>[24x]MSQSGEDLHSPTYLSWRKLQLSRAKLKASSWTSALLSGFAMVAMVEVQLDHDTNVPPGMLIAFAICTTLLVAVHMLALMISTCILPNIETVSNLHSISLVHESPHERLHWYIETAWAFSTLLGLILFLLEIAILCWVKFYDLSPPAAWSATVVLIPVMIIFMAFAIHFYRSLVSHKYEVTVSGIRELEMLKEQMEQDHLEHHNNIRNNGEGEEF

Orai was identified as the protein that forms the channel’s pore and STIM was identified as its regulator. The channel is activated by the depletion of Ca2+ from the endoplasmic reticulum (ER), and as such it was characterized as the calcium release-activated calcium (CRAC) channel responsible for store-operated calcium entry (SOCE) before the molecular components were known. The channel is formed from an assembly of six Orai subunits that surround a single ion pore, which is perpendicular to the plasma membrane in a cellular setting. Each Orai subunit contains four transmembrane helices (M1-M4) and a cytosolic M4-ext helix.

The K163W mutation corresponds to R91W in human Orai1, which is a loss of function mutation that causes a severe combined immune deficiency-like disorder. To exclude the possibility that the crystal contacts in the H206A Oraicryst structure were responsible for the conformational changes we observed in the pore, we determined the structures of wild-type (WT) Oraicryst and K163W Oraicryst grown in the same crystal form (I41). Well-defined electron density maps of WT and K163W Oraicryst were obtained using non-crystallographic symmetry averaging of modest (6.9 and 6.1 Å, respectively) resolution diffraction data in the same manner as for the H206A Oraicryst structure. The structures of WT and K163W Oraicryst reveal an ‘unlatched-closed’ conformation of the channel that resembles a hybrid of the quiescent and open conformations: the ion pores are closed as in the quiescent conformation but the M4/M4-ext regions have conformations like those observed in the H206A Oraicryst structure. The conformation of the M1-M4a portion of the channel, however, is like the quiescent conformation, and as such, the pores of WT and K163W Oraicryst are closed and indistinguishable from the pore in the structure of the quiescent conformation. As in the quiescent conformation, anomalous difference electron density for an iron complex is observed in the basic region of the pore in the unlatched-closed conformation. The density is positioned roughly in the center of the basic region in the structure of WT Oraicryst and located in the lower portion of it in the structures of the K163W mutant, which removes the top ring of basic residues from the pore. The K163W mutation has no other apparent effect, and this is analogous to observations from structures of the quiescent conformation with and without the K163W mutation. Congruently, we observe that the corresponding K163W mutant of Drosophila Orai can adopt an unlatched conformation with a closed pore. The structures of the unlatched-closed conformation reveal that release of the latches does not necessarily open the pore: the pore is closed despite the M4b and M4-ext helices adopting the same conformation that they do in the H206A structure.> MAPQIRSRSLAAQEPASVLEEARLRLHVSAVPESLPCREQEFQDIYNFVESKLLDHTGGCMYISGVPGTGKTATVHEVIRCLQQAAQANDVPPFQYIEVNGMKLTEPHQVYVQILQKLTGQKATANHAAELLAKQFCTRGSPQETTVLLVDELDLLWTHKQDIMYNLFDWPTHKEARLVVLAIANTMDLPERIMMNRVSSRLGLTRMCFQPYTYSQLQQILRSRLKHLKAFEDDAIQLVARKVAALSGDARRCLDICRRATEICEFSQQKPDSPGLVTIAHSMEAVDEMFSSSYITAIKNSSVLEQSFLRAILAEFRRSGLEEATFQQIYSQHVALCRMEGLPYPTMSETMAVCSHLGSCRLLLVEPSRNDLLLRVRLNVSQDDVLYALKDE;> MSKPELKEDKMLEVHFVGDDDVLNHILDREGGAKLKKERAQLLVNPKKIIKKPEYDLEEDDQEVLKDQNYVEIMGRDVQESLKNGSATGGGNKVYSFQNRKHSEKMAKLASELAKTPQKSVSFSLKNDPEITINVPQSSKGHSASDKVQPKNNDKSEFLSTAPRSLRKRLIVPRSHSDSESEYSASNSEDDEGVAQEHEEDTNAVIFSQKIQAQNRVVSAPVGKETPSKRMKRDKTSDLVEEYFEAHSSSKVLTSDRTLQKLKRAKLDQQTLRNLLSKVSPSFSAELKQLNQQYEKLFHKWMLQLHLGFNIVLYGLGSKRDLLERFRTTMLQDSIHVVINGFFPGISVKSVLNSITEEVLDHMGTFRSILDQLDWIVNKFKEDSSLELFLLIHNLDSQMLRGEKSQQIIGQLSSLHNIYLIASIDHLNAPLMWDHAKQSLFNWLWYETTTYSPYTEETSYENSLLVKQSGSLPLSSLTHVLRSLTPNARGIFRLLIKYQLDNQDNPSYIGLSFQDFYQQCREAFLVNSDLTLRAQLTEFRDHKLIRTKKGTDGVEYLLIPVDNGTLTDFLEKEEEEA;> MATSSMSKGCFVFKPNSKKRKISLPIEDYFNKGKNEPEDSKLRFETYQLIWQQMKSENERLQEELNKNLFDNLIEFLQKSHSGFQKNSRDLGGQIKLREIPTAALVLGVNVTDHDLTFGSLTEALQNNVTPYVVSLQAKDCPDMKHFLQKLISQLMDCCVDIKSKEEESVHVTQRKTHYSMDSLSSWYMTVTQKTDPKMLSKKRTTSSQWQSPPVVVILKDMESFATKVLQDFIIISSQHLHEFPLILIFGIATSPIIIHRLLPHAVSSLLCIELFQSLSCKEHLTTVLDKLLLTTQFPFKINEKVLQVLTNIFLYHDFSVQNFIKGLQLSLLEHFYSQPLSVLCCNLPEAKRRINFLSNNQCENIRRLPSFRRYVEKQASEKQVALLTNERYLKEETQLLLENLHVYHMNYFLVLRCLHKFTSSLPKYPLGRQIRELYCTCLEKNIWDSEEYASVLQLLRMLAKDELMTILEKCFKVFKSYCENHLGSTAKRIEEFLAQFQSLDAETKEEEDASGSQPKGLQKTDLYHLQKSLLEMKELRRSKKQTKFEVLRENVVNFIDCLVREYLLPPETQPLHEVVYFSAAHALREHLNAAPRIALHTALNNPYYYLKNEALKSEEGCIPNIAPDICIAYKLHLECSRLINLVDWSEAFATVVTAAEKMDANSATSEEMNEIIHARFIRAVSELELLGFIKPTKQKTDHVARLTWGGC;> MSSRKSKSNSLIHTECLSQVQRILRERFCRQSPHSNLFGVQVQYKHLSELLKRTALHGESNSVLIIGPRGSGKTMLINHALKELMEIEEVSENVLQVHLNGLLQINDKIALKEITRQLNLENVVGDKVFGSFAENLSFLLEALKKGDRTSSCPVIFILDEFDLFAHHKNQTLLYNLFDISQSAQTPIAVIGLTCRLDILELLEKRVKSRFSHRQIHLMNSFGFPQYVKIF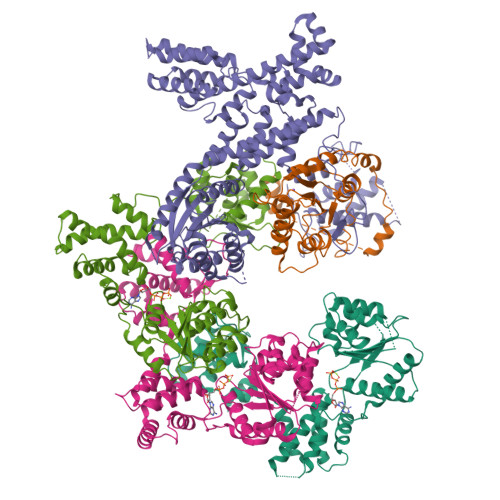KEQLSLPAEFPDKVFAEKWNENVQYLSEDRSVQEVLQKHFNISKNLRSLHMLLMLALNRVTASHPFMTAVDLMEASQLCSMDSKANIVHGLSVLEICLIIAMKHLNDIYEEEPFNFQMVYNEFQKFVQRKAHSVYNFEKPVVMKAFEHLQQLELIKPMERTSGNSQREYQLMKLLLDNTQIMNALQKYPNCPTDVRQWATSSLSWL;> MPHLENVVLCRESQVSILQSLFGERHHFSFPSIFIYGHTASGKTYVTQTLLKTLELPHVFVNCVECFTLRLLLEQILNKLNHLSSSEDGCSTEITCETFNDFVRLFKQVTTAENLKDQTVYIVLDKAEYLRDMEANLLPGFLRLQELADRNVTVLFLSEIVWEKFRPNTGCFEPFVLYFPDYSIGNLQKILSHDHPPEYSADFYAAYINILLGVFYTVCRDLKELRHLAVLNFPKYCEPVVKGEASERDTRKLWRNIEPHLKKAMQTVYLREISSSQWEKLQKDDTDPGQLKGLSAHTHVELPYYSKFILIAAYLASYNPARTDKRFFLKHHGKIKKTNFLKKHEKTSNSLLGPKPFPLDRLLAILYSIVDSRVAPTANIFSQITSLVTLQLLTLVGHDDQLDGPKYKCTVSLDFIRAIARTVNFDIIKYLYDFL We verified that the Mimivirus and M. chilensis predicted PAPs were able to perform polyadenylation. These proteins were not only active, but also intrinsically self-processive, generating >700 nucleotides long polyA tails. To elucidate the molecular basis of this processivity we determined the Mimivirus and M. chilensis PAP crystallographic 3D structures, which revealed two topologically identical subdomains with a nucleotidyltransferase fold. Thus, while other PAPs form heterodimers with processivity factors, the Mimivirus and M. chilensis PAP become processive upon homodimerization.

Since they shared the same characteristic features, we will refer to the highest resolution structure of Mg561. As observed in solution (see later), the Mg561 crystal structure reveals a very stable homodimer with an almost perfect two-fold symmetry axis (179°) and a 3200 Å2 buried surface area upon dimerization. The dimer structure highlights a large tunnel at the interface between the two monomers. The N-terminal domain (D1) encompasses an extended strand followed by a long helix (α1) bent at the P28 residue. In each monomer, this helix creates a domain swap, and makes contact with the D4 loop located between α13 and β16 and the α7 helix of the D2 domains of the other monomer to form the dimer structure. The third domain (D3) of the Mg561 structure surprisingly mimics the catalytic domain topology leading to an internal symmetry between the D2 and D3 domains (rotation of 162°, 2.4 Å translation and Cα-rmsd > 2.0 Å). Two of the three catalytic residues (F286, E288, K342) are replaced by non-canonical residues in D3, and an even longer insertion within the helix-turn motif (37 amino-acids) of the NT-like subdomain is present. The interaction with the D3 domain is stabilized by a conserved disulfide bridge (C350-C426) connecting the beginning of the β14 strand and the β16 strand in the D4 domain. Electrostatic potential calculations highlight intensely positively charged grooves on each side of the entrance of the central tunnel, which is contributed mostly by the positively charged D4 domains and to a lesser extent by the D2, D3 domains. RNAs could therefore interact with the PAP through the positively charged grooves and reach the catalytic site through the 10 Å diameter wide central tunnel making the two catalytic sites accessible for a ssRNA molecule.

>GPGSSENRNRKLSYQEYYVDGDYEEVRKKLPEIIKQARIKASQVMEPTIYEKRVVMEIIKDFIRDKGRKVYGGTALNETIKKKNPEDAIYDSYLFSDIEFYSPTPVPDLKELCDILYHKGYDPVQGKEAQHEETYSIFVNLQLYCDITYVPTKVYHGIKTIEIDGINYTHPHFMLIDYLRMINQPLTAAEQRWEKAFDRMYVLLKNYPMEKYDNSMRITSPRDDIQMYIGKVKSEFMKIPEIQESCLISGFDAYNFFIRHAMGDRKVEQMARIKNDYNSLKNFITVLPFMELISVKYKDTVEKLYNFLREKVVNPDLITIDEYFPLFQFTGYSVSINYDGIPIVKVYEADGYCVPDIKTTSGYRYVSYQYILMIMYISKFKAHLDKNKEMYFNYGIAISNLVQARNSYLNQKNIGVINDTVFSEFRIGCIGTTVSYTRMSRLRMLEKKKQGKVIQFVYTPKQYFSQTPEQQNNFDESMKKYRFKNTSGNKITIPKNLLFKIDERGNISEEISTEEAYITEDTTSINTTTDINTN[2x]> MLGAVEGPRWKQAEDIRDIYDFRDVLGTGAFSEVILAEDKRTQKLVAIKCIAKEALEGKEGSMENEIAVLHKIKHPNIVALDDIYESGGHLYLIMQLVSGGELFDRIVEKGFYTERDASRLIFQVLDAVKYLHDLGIVHRDLKPENLLYYSLDEDSKIMISDFGLSKMEDPGSVLSTACGTPGYVAPEVLAQKPYSKAVDCWSIGVIAYILLCGYPPFYDENDAKLFEQILKAEYEFDSPYWDDISDSAKDFIRHLMEKDPEKRFTCEQALQHPWIAGDTALDKNIHQSVSEQIKKNFAKSKWKQAFNATAVVRHMRKLQ

When activated, CaM binds to and stimulates the activities of a family of Ca2+/CaM-dependent serine/threonine protein kinases (CaMKs), thereby regulating their functions. However, the regulation mechanism of CaMKI remains elusive. Here we report four crystal structures of three truncation variants of human CaMKIα, namely CaMKI320 (residues 1–320), CaMKI315 (residues 1–315), and CaMKI293 (residues 1–293), which correspond to the aforementioned three truncation forms of CaMKI, respectively. The catalytic core of CaMKI takes a canonical bilobate architecture, with the N-terminal lobe (N lobe) consisting of five antiparallel β-strands and a prominent helix named helix αC and the C-terminal lobe (C lobe) comprised primarily of α-helices.

In contrast, in our CaMKI320, the P-loop takes a canonical conformation, the C-terminus of the regulatory region (residues 300–320) is undetected, and the nucleotide-binding site is amenable to nucleotide binding. More intriguingly, the C-terminal part of the activation segment encompassing residues Pro171 to Thr181 assumes a unique helical conformation (designated as helix αT) with well-defined electron density (an average B factor of 39.8 Å2) and the DFG motif at the N-terminal part of the activation segment takes an “in” conformation. The rare helical conformation of αT is stabilized by the hydrophilic and hydrophobic interactions within the activation segment and with the surrounding secondary structure elements including helices αEF and αG and the αEF-αF loop. Specifically, the hydroxyl of Thr177 (the phosphorylation site of the activation segment) forms hydrogen-bonding interactions indirectly with the hydroxyl of Tyr195 (a strictly conserved residue on the αEF-αF loop) and the main-chain carbonyl of Met168 via a water molecule, and the hydroxyl of Ser173 forms a hydrogen bond with the main-chain carbonyl of Lys167. In the apo CaMKI320, Lys49 interacts with Asp162 and Phe163 of the DFG motif of the activation segment. Concurrently, helix αC is rotated outward and Glu66 points its side chain away from the catalytic site, making it impossible to interact with Lys49. Whereas in CaMKI320, the activation segment including helix αT and the β8-αT loop occupies part of the catalytic site. Although unphosphorylated, the side chain of Thr177 (equivalent to Thr309 of Akt/PKB) is oriented inwards and forms interactions with the surrounding residues to stabilize the specific conformation of the activation segment, shielding it from surface exposure and hence from CaMKK phosphorylation.> EDISEPPLHDFYCSRLLDLVFLLDGSSRLSEAEFEVLKAFVVDMMERLRISQKWVRVAVVEYHDGSHAYIGLKDRKRPSELRRIASQVKYAGSQVASTSEVLKYTLFQIFSKIDRPEASRIALLLMASQEPQRMSRNFVRYVQGLKKKKVIVIPVGIGPHANLKQIRLIEKQAPENKAFVLSSVDELEQQR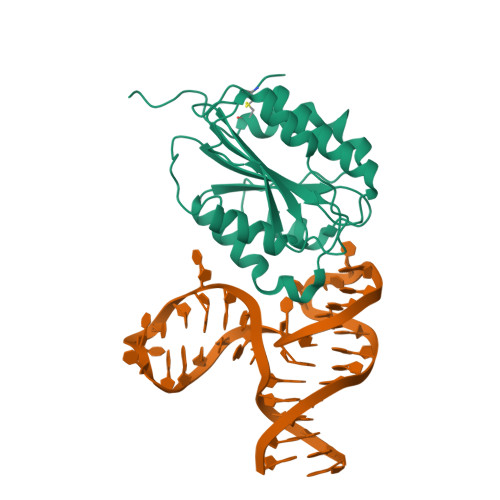DEIVSYLCDLAPEAPPPT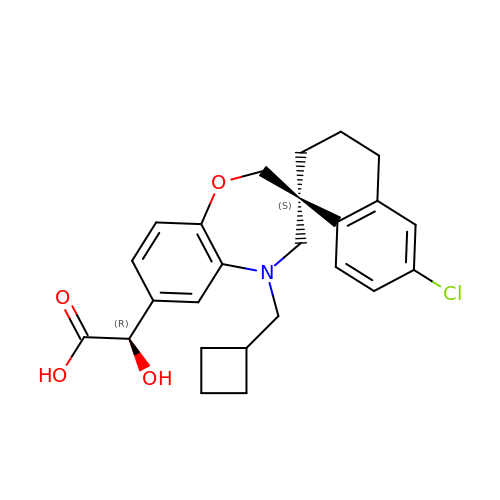(2R)-[(3S)-6'-chloro-5-(cyclobutylmethyl)-3',4,4',5-tetrahydro-2H,2'H-spiro[1,5-benzoxazepine-3,1'-naphthalen]-7-yl](hydroxy)acetic acid | C25 H28 Cl N O4 | COMWCPYAPXFWGY-NOZRDPDXSA-N> VVGGTRAAQGEFPFMVRLSMGCGGALYAQDIVLTAAHCVSGSGNNTSITATGGVVDLQSSSAVKVR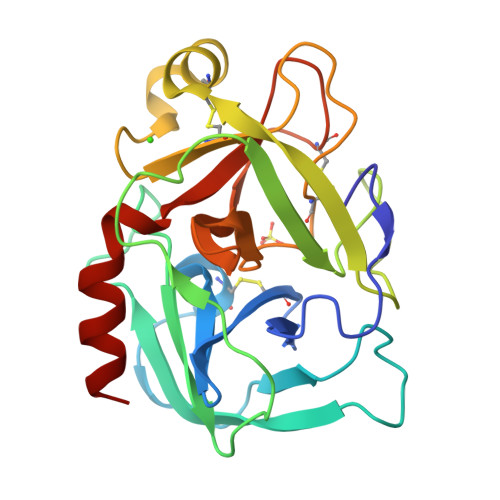STKVLQAPGYNGTGKDWALIKLAQPINQPTLKIATTTAYNQGTFTVAGWGANREGGSQQRYLLKANVPFVSDAACRSAYGNELVANEEICAGYPDTGGVDTCQGDSGGPMFRKDNADEWIQVGIVSWGYGCARPGYPGVYTEVSTFASAIASAARTL URIDINE-5'-DIPHOSPHATE | C9 H14 N2 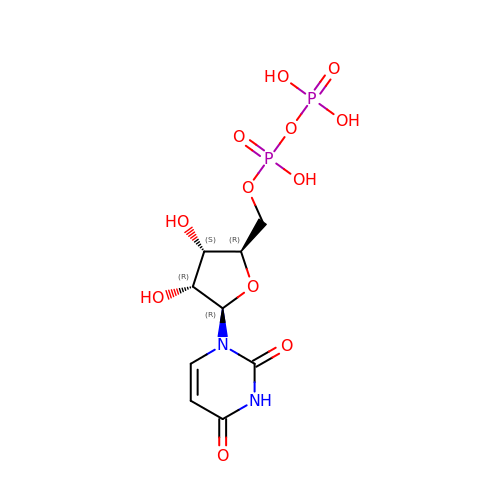O12 P2 | XCCTYIAWTASOJW-XVFCMESISA-N> MVKVIFFDLDDTLVDTSKLAEIARKNAIENMIRHGLPVDFETAYSELIELIKEYGSNFPYHFDYLLRRLDLPYNPKWISAGVIAYHNTKFAYLREVPGARKVLIRLKELGYELGIITDGNPV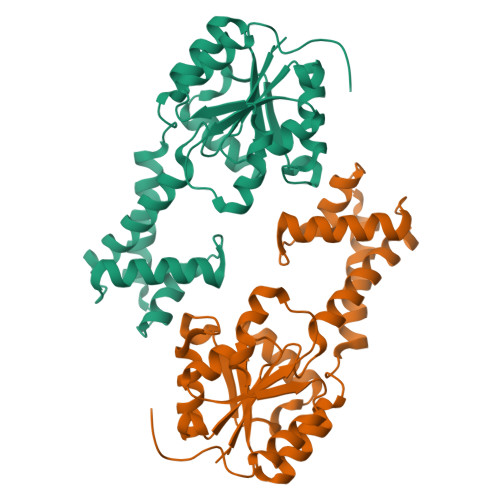KQWEKILRLELDDFFEHVIISDFEGVKKPHPKIFKKALKAFNVKPEEALMVGDRLYSDIYGAKRVGMKTVWFRYGKHSERELEYRKYADYEIDNLESLLEVLARESSSNKKVHPPRQQI> APNDQHYREQWHYFDRYGVKADKVWDMGFTGQNVVVAVVDTGILHHRDLNANVLPGYDFISNSQISLDGDGRDADPFDEGDWFDNWACGGYPDPRKERSDSSWHGSHVAGTIAAVTNNRIGVAGVAYGAKVVPVRALGRCGGYDSDISDGLYWAAGGRIAGIPENRNPAKVINMSLGSDGQCSYNAQTMIDRATRLGALVVVAAGNENQNASNTWPTSCNNVLSVGATTSRGIRASFSNYGVDVDLAAPGQDILSTVDSGTRRPVSDAYSFMAGTSMATPHVSGVAALVISAANSVNKNLTPAELKDVLVSTTSPFNGRLDRALGSGIVDAEAAVNSVLG

Dichelobacter nodosus is a Gram negative, anaerobic rod that is the principal causative agent of ovine footrot, a debilitating disease of the hoof of ruminants. In strains that cause virulent footrot these proteases are called acidic protease isoenzymes 2 and 5 from virulent strains (AprV2 and AprV5) and basic protease from virulent strains (BprV). All of these proteases are synthesised as inactive precursors with an N-terminal pre-pro-region, a serine protease domain and a C-terminal domain of unknown function. AprV2 adopts a subtilisin-like fold consisting of a curved six-stranded parallel beta sheet sandwiched between two and five alpha helices.

To investigate how the single amino acid difference (Y92R) between the active forms of AprV2 and AprB2 alters the substrate specificity of AprB2 we determined the crystal structures of AprV2 and AprB2 to 2.0 Å and 1.7 Å, respectively. The two structures were very similar (RMSD of 0.28 Å for 339 Cα) and therefore we will describe the structure with reference to AprV2. The proteases have two disulphide bonds, Cys89-Cys141 and Cys183-Cys220 and three calcium binding sites. The most striking feature of the substrate binding site is a large, elongated S1 binding pocket, which is lined by residues 177–180, 204–208, 215 and 218, and appears capable of accommodating bulky side-chains such as phenylalanine. This finding is consistent with previous studies, which have shown that AprV2 preferentially cleaves after phenylalanine or leucine residues. Comparison with other subtilisin-like proteases reveals several major insertions (termed I1-I4) in the loops that surround the active site cleft. Most notable is the large well ordered I2 loop (residues 82–102) that is tethered to the subtilisin-like fold by a disulphide bond between Cys141 and Cys89. The loop is well defined in the electron density, with low B-factors, suggesting that it has limited mobility in the crystal structure. However, the apparent stability of the I2 loop is likely to arise from crystal packing and it is uncertain if this conformation would be favoured in solution. We therefore propose that the I2 loop functions as an exosite, mediating the formation of a stable enzyme-substrate complex.>[2x]MAAHLSYGRVNLNVLREAVRRELREFLDKCAGSKAIVWDEYLTGPFGLIAQYSLLKEHEVEKMFTLKGNRLPAADVKNIIFFVRPRLELMDIIAENVLSEDRRGPTRDFHILFVPRR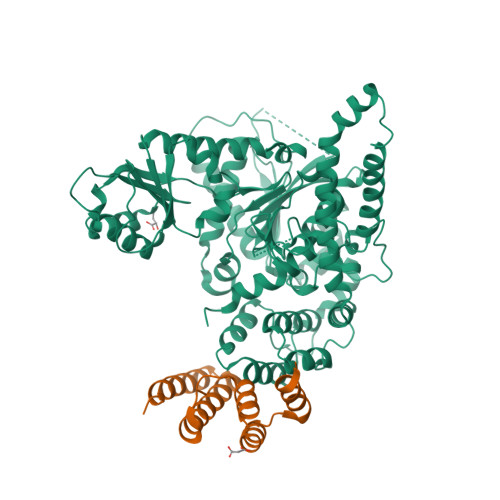SLLCEQRLKDLGVLGSFIHREEYSLDLIPFDGDLLSMESEGAFKECYLEGDQTSLYHAAKGLMTLQALYGTIPQIFGKGECARQVANMMIRMKREFTGSQNSIFPVFDNLLLLDRNVDLLTPLATQLTYEGLIDEIYGIQNSYVKLPPEKFAPKKQGDGGKDLPTEAKKLQLNSAEELYAEIRDKNFNAVGSVLSKKAKIISAAFEERHNAKTVGEIKQFVSQLPHMQAARGSLANHTSIAELIKDVTTSEDFFDKLTVEQEFMSGIDTDKVNNYIEDCIAQKHSLIKVLRLVCLQSVCNSGLKQKVLDYYKREILQTYGYEHILTLHNLEKAGLLKPQTGGRNNYPTIRKTLRLWMDDVNEQNPTDISYVYSGYAPLSVRLAQLLSRPGWRSIEEVLRILPGPHFEERQPLPTGLQKKRQPGENRVTLIFFLGGVTFAEIAALRFLSQLEDGGTEYVIATTKLMNGTSWIEALMEKPFHHHHHHHHHH;> GPHMERIEGRVAALQTAADAFYKAKNEFAAKATEDQMRLLRLQRRLEDELGGQFLDLSLHDTVTTLILGGHNKRAEQLARDFRIPDKRLWWLKLTALAD>DPFTMQVSQYLYQNAQSIWGDCISHPFVQGIGRGTLERDKFRFYIIQDYLYLLEYAKVFALGVVKACDEAVMREFSNAIQDILNNEMSIHNHYIRELQITQKELQNACPTLANKSYTSYMLAEGFKGSIKEVAAAVLSCGWSYLVIAQNLSQIPNALEHAFYGHWIKGYSSKEFQACVNWN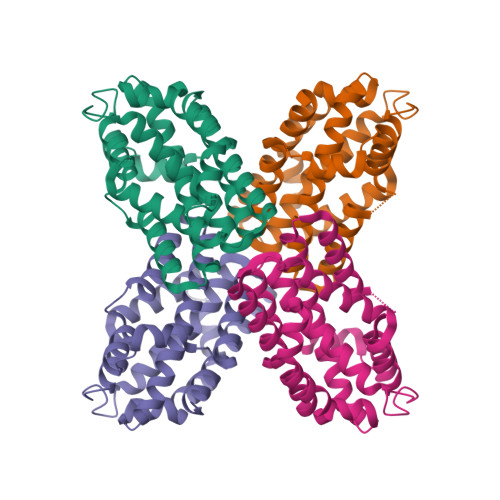INLLDSLTLASSKQEIEKLKEIFITTSEYEYLFWDMAYQS[2x]>[2x]MDAVKKAILGEVLEEEEA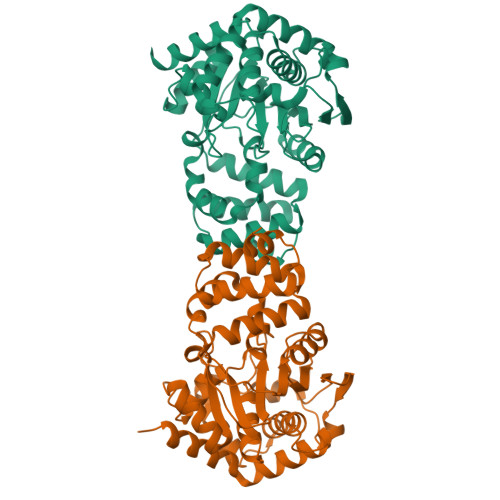YEVMRALMAGEVSPVRAAGLLVALSLRGERPHEIAAMARAMREAARPLRVHRRPLLDIVGTGGDGKGLMNLSTLAALVAAAGGVAVAKHGNRAASSRAGSADLLEALGVDLEAPPERVGEAIEELGFGFLFARVFHPAMRHVAPVRAELGVRTVFNLLGPLTNPAGADAYVLGVFSPEWLAPMAEALERLGARGLVVHGEGADELVLGENRVVEVGKGAYALTPEEVGLKRAPLEALKGGGPEENAALARRLLKGEEKGPLADAVALAAGAGFYAAGKTPSLKEGVALAREVLASGEAYLLLERYVAFLRA>[3x]MGSDKIHHHHHHMMKKIEEARTFISERTNLSPDILIILGSGFGPFIEKVEDPVIIDYKDIPHFPQPTVEGHSGKLVFG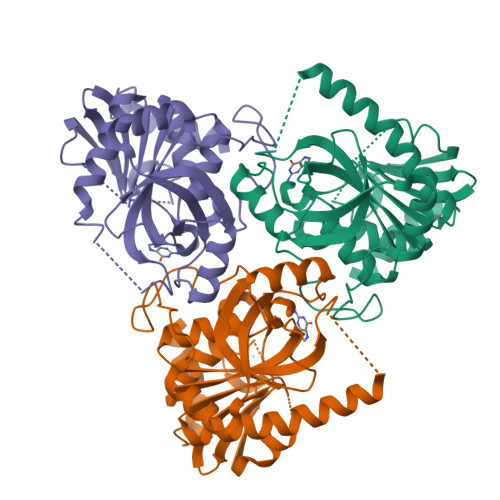RISDKPVMIMAGRFHLYEGHDPATVAFPVYLAKYVGVKGVVVTNAAGAINPEFKPGEIILVRDIINFMFRNPLRGPNDEKIGPRFPDMSSVVDPEWARKIQERLSLKEGVYIGVLGPSYETPAEIRVFEKLGADLVGMSTVPEVIAAKHCGLKVVVFSCVTNMAAGITHGRLSHEEVVRTTKMAQGKIEKALTTAVEVF>MDNKTYEISSAEWEVMNIIWMKKYASANNIIEEIQMQKDWSPKTIRTLITRLYKKGFIDRKKDNKIFQYYSLVEESDIKYKTSKNFINKVYKGGFNSLVLNFVEKEDLSQDEIEELR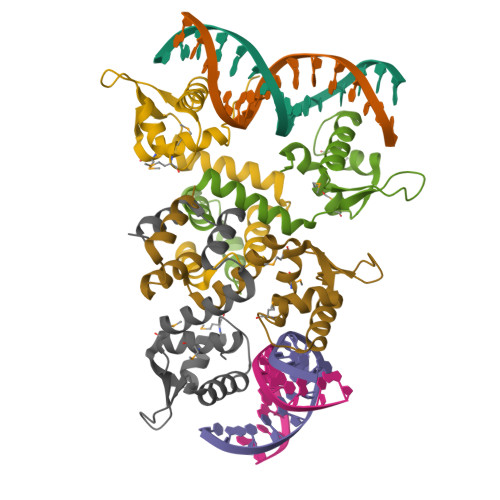NILNKK[4x]> MGSSHHHHHHSQDPLEVLFQGPEFMSAIKPDMKIKLRMEGNVNGHHFVIDGDGTGKPFEGKQSMDLEVKEGGPLPFAFDILTTAFHYGNRVFAKYPDNIQDYFKQSFPKGYSWERSLTFEDGGICNARNDITMEGDTFYNKVRFYGTNFPANGPVMQKKTLKWEPSTEKMYVRDGVLTGDIEMALLLEGNAHYRCDFRTTY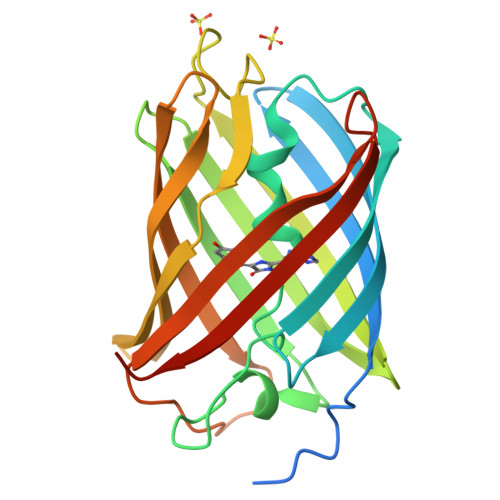KAKEKGVKLPGAHFVDHCIEILSHDKDYNKVKLYEHAVAHSGLPDNARR[(3~{R})-4-[2-[2-[[3-(2-azanyl-6-chloranyl-pyrimidin-4-yl)-1-[bis(fluoranyl)methyl]pyrazol-4-yl]methyl]phenoxy]ethyl]morpholin-3-yl]methanol 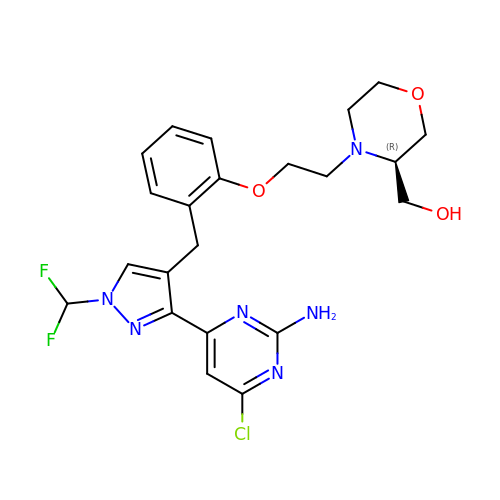| C22 H25 Cl F2 N6 O3 | XVGSKZXXLKUEIO-MRXNPFEDSA-N The redox-responding transcription factor PpsR (photopigment suppression) from Rhodobacter sphaeroides is such a multi-PAS domain-containing protein. PpsR possesses three PAS domains (designated N-domain, PAS1 and PAS2) and a highly conserved glutamine-rich linker (Q-linker) as well as a C-terminal helix–turn–helix (HTH) DNA-binding motif. PpsR acts as a repressor of photosynthesis and tetrapyrrole-biosynthesis gene expression by binding to palindromic DNA sequences (TGTc-N10-gACA) present in the promoter region of PpsR-regulated genes. Additionally, the function of PpsR is regulated in a blue-light- and oxygen-dependent manner by the antirepressor AppA that, together with PpsR and its cognate DNA, is able to form a light-sensitive ternary AppA–PpsR2–DNA complex.

Phases for PpsRN-Q-PAS1 were obtained by MR using the PpsRQ-PAS1 dimer as a search model. Since the dimer arrangement of the PAS1 domain was virtually identical in both crystal forms, we obtained excellent phases and could model the remaining parts of the Q-linker and the N-domain into the electron-density map. The PpsRN-Q-PAS1 dimer has a barbell-like quaternary structure with a protomer crossing along a central imperfect dyad axis. Owing to the protomer crossing, the N-­domain and PAS1 domain of a single protomer are located on opposite sides of the dyad axis. The functional relevance of the observed dimer architecture is supported by a large number of contacts, which lead to a total BSA of 6180 Å2. The PpsRN-Q-PAS1 structure also allowed the identification of an additional PAS domain in the N-terminal part of PpsR, which was predicted based on sequence information from some PpsR homologues. The PAS core is N-­terminally flanked by a helix (αN), which again corresponds to a classical PAS N-cap and constitutes a central part of the N-domain dimer interface, in analogy to the N-cap of PAS1. The highly conserved Q-linkers form a ∼57 Å long coiled-coil-like structure which connects the N-domain dimers to the PAS1 dimers. However, neither tailing nor a reduction in the elution volume of the eluting peak was observed during PpsRN-Q-PAS1 purification, suggesting that PpsRN-Q-PAS1 is not able to form tetramers even at high concentrations. Additionally, the observed PpsRN-Q-PAS1 dimer organization appears to resemble a general architecture for the connection of PAS modules with a variety of effector or sensory domains.

>[2x]GAMGMGLAGGSLPSLAPDLVRDLIATAADISLLVSQEGVVREVMANPHHPSFGQLSEWEGRPLEEVLTAESVAKFRLRSEGLEPGRGSVAVELNHIDPRSFEFPIRYILHRLPADRSILMLGRDLRPIAEVQQQLVAAQLAMERDYETQREMETRYRVVLDVSRDPMVLVSMSTGRIVDLNSAAGLLLGGVRQDLLGAAIAQEFEGRRRGEFMETMTNLAATESAAPVEVLARRSQKRLLVVPRVFRAAGERLLLCQIDPAD>MEELQDDYEDMMEENLEQEEYEDPDIPESQMEEPAAHDTEATATDYHTTSHPGTHKVYVELQELVMDEKNQELRWMEAARWVQLEENLGENGAWGRPHLSHLTFWSLLELRRVFTKGTVLLDLQETSLAGVANQLLDRFIFEDQIRPQDREELLRALLLKHSHAGELEALGGVKPAVLTRSGDPSQPLLPQHSSLETQLFCEQGDGGTEGHSPSGILEKIPPDSEATLVLVGRADFLEQPVLGFVRLQEAAELEAVELPVPIRFLFVLLGPEAPHIDYTQLGRAAATLMSERVFRIDAYMAQSRGELLHSLEGFLDCSLVLPPTDAPSEQALLSLVPVQRELLRRRYQSSPAKPDSSFYKGLDLNGGPDDPLQQTGQLFGGLVRDIRRRYPYYLSDITDAFSPQVLAAVIFIYFAALSPAITFGGLLGEKTRNQMGVSELLISTAVQGILFALLGAQPLLVVGFSGPLLVFEEAFFSFCETNGLEYIVGRVWIGFWLILLVVLVVAFEGSFLVRFISRYTQEIFSFLISLIFIYETFSKLIKIFQDHPLQKTYNYNVLMVPKPQGPLPNTALLSLVLMAGTFFFAMMLRKFKNSSYFPGKLRRVIGDFGVPISILIMVLVDFFIQDTYTQKLSVPDGFKVSNSSARGWVIHPLGLRSEFPIWMMFASALPALLVFILIFLESQITTLIVSKPERKMVKGSGFHLDLLLVVGMGGVAALFGMPWLSATTVRSVTHANALTVMGKASTPGAAAQIQEVKEQRISGLLVAVLVGLSILMEPILSRIPLAVLFGIFLYMGVTSLSGIQLFDRILLLFKPPKYHPDVPYVKRVKTWRMHLFTGIQIICLAVLWVVKSTPASLALPFVLILTVPLRRVLLPLIFRNVELQCLDADDAKATFDEEEGRDEYDEVAMPV[2x];>[2x]MGQALGIKSCDFQAARNNEEHHTKALSSRRLFVRRGQPFTIILYFRAPVRAFLPALKKVALTAQTGEQPSKINRTQATFPISSLGDRKWWSAVVEERDAQSWTISVTTPADAVIGHYSLLLQVSGRKQLLLGQFTLLFNPWNREDAVFLKNEAQRMEYLLNQNGLIYLGTADCIQAESWDFGQFEGDVIDLSLRLLSKDKQVEKWSQPVHVARVLGALLHFLKEQRVLPTPQTQATQEGALLNKRRGSVPILRQWLTGRGRPVYDGQAWVLAAVACTVLRCLGIPARVVTTFASAQGTGGRLLIDEYYNEEGLQNGEGQRGRIWIFQTSTECWMTRPALPQGYDGWQILHPSAPNGGGVLGSCDLVPVRAVKEGTLGLTPAVSDLFAAINASCVVWKCCEDGTLELTDSNTKYVGNNISTKGVGSDRCEDITQNYKYPEGSLQEKEVLERVEKEKMEREKDNGIRPPSLETASPLYLLLKAPSSLPLRGDAQISVTLVNHSEQEKAVQLAIGVQAVHYNGVLAAKLWR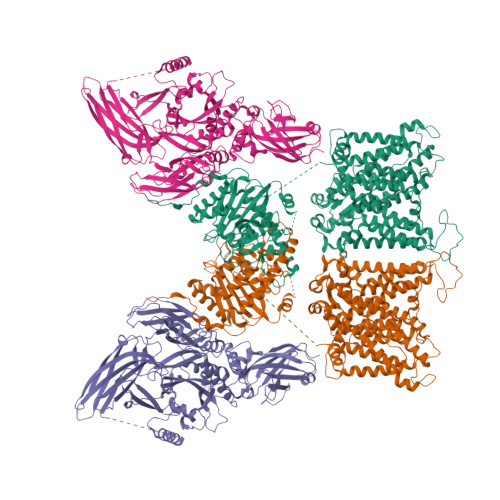KKLHLTLSANLEKIITIGLFFSNFERNPPENTFLRLTAMATHSESNLSCFAQEDIAICRPHLAIKMPEKAEQYQPLTASVSLQNSLDAPMEDCVISILGRGLIHRERSYRFRSVWPENTMCAKFQFTPTHVGLQRLTVEVDCNMFQNLTNYKSVTVVAPELSA> GMISLNNRLTTVSRFLKQGTIADIGSDHAYLPIYAIQNHLCECGIAGEVIQGPFQAAVKNVAANQLVDRIDVRLGDGLSVIQPEDVIDNITICGMGGPLIAKILKDGQDKLSQHPRLILQSNIQTENLRQTLQQLNYEIIDEIIMEEKGHIYEIVVAEYSTELIELSSDELKFGPKLLNNKNEYFIKKWQRELEALYHIKSKLNTEQHHQRLAQINDEIAVIERV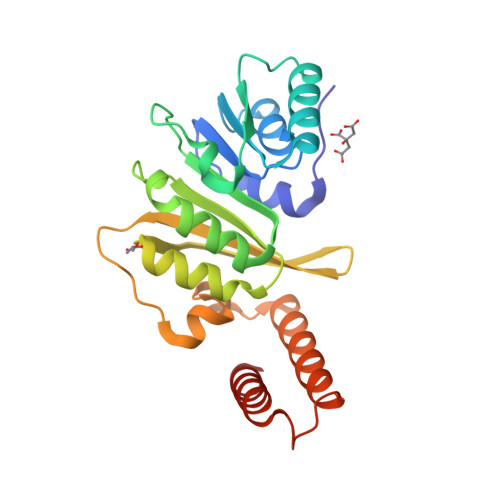L>[2x]PSVYDAAAQLTADVKKDLRDSWKVIGSDKKGNGVALVTTLFADNQETIGYFKRLGDVSQGMANDKLRGHSITLMYALQNFIDQLDNPDDLVCVVEKFAVNHITR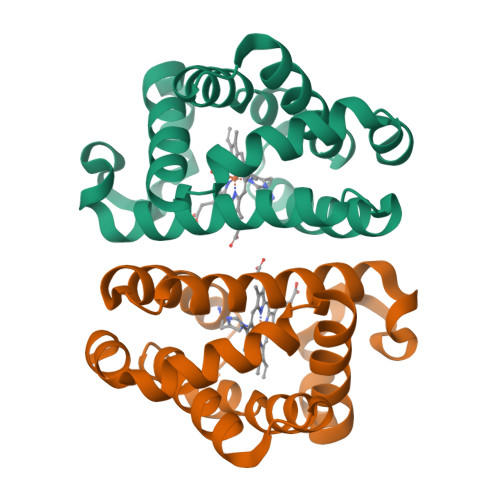KISAAEFGKINGPIKKVLASKNFGDKYANAWAKLVAVVQAAL>MVKVDLESKRYGEKLKEVFLMLDNNVVECIKEITESSRNGKLVFFVGAGVSTLSDYPQWWRLVDKYHEELYGSPKKGNYSSDEYLRIPQIFYNVKGEMAFDGILKDFFQVDKPTNPIHDKILAMNPAHVITTAYDNLIDTACWKRGKYFSVISAEEDVANATSSRYLLKVAGDFRKGFKGENVVLKEDDYLNYDQNYPLISNLMKTIIATHTIVFIGYGLGDYNINMLLNWVRKLQKDSFHKPFFIRTDPSPIENETLIYYENKGLRIIDAASLIDSNEYDYLERYSAVMDLLIESQENKFITKDDEVIDYIYGKISPLFALQYIRKIDLKHVFEYDYHFEVNGTVVRHKNKGFGYMERFFELKESCDERSKLSKKQYERFNALFNFFEKNGVICMAKDAGTLNTSIEINSLAYHGKYDVMKKFIEEQSVSIEDDYKKAFFLACLGRWEESYDLYSNIILNSIDESNGCVYYLSQINRYRIYQSITQAVTQFNGLGLLTFGRHYKPFTDEFLARIEREMTNFNIDDLFNGMPFEFQKKYKILEFLSDNQFLYDDTVKLFELTNKVRSEMSEGSYSFGMSSDIVVLLRLYDNLRFLYENCLWSVSFHEFHQYIRNSMSLLIEKAEYERTRDIDELGFSFFGKKSGFFMEYYDFVNISRHFKIDDIKNLERSCSIDKIRFGEQEKIEEYLVGIAEEITKQFSANGMNVVFYTQFISEAKAALYFAKYVKLSEEGLGKIVKALLFYFPERDLDIGKRYVWLERLTKCNELPKSIISIIDDFLVLQAEKHIDQNYSEVSSNGLYSRDYGALIKHFEKNFISKRLSEITLCLTQDKQKQIDFLFKLLPLLSTNAKSHLLSFKSVENINDLMNGIRIGLIDEFTPEHEELIIEYLETRKVNYIVEKEKGIQTFSSNDYMSTFGIWYFLEEINNSKMEEFIGMDDQYDFFVDPENFDYKKFIPSWLKNYNDKLLGKIAGNKHMKHHVIEVLKERVKNSNDKRYLEILMNYFI[4x];>MKTVIQDTADVYFK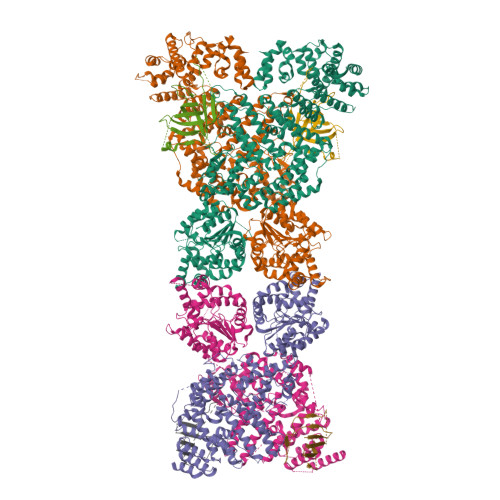RKSDGKLVFTAEAQTASFSQAISEEKLRGGIGNKPLYILKSEKEINLTVKNAFFDLEWLAMTQGETIQEETKVKVFDREHGLIVDDTNKVTLKGKPVSDVTFYNKKGLTYKIAVSTDGTYTIPTAFAAAKDKLTAVYQIEKVGRRLAIKASKFSERYEVEYRTIAYNPDTEEVYSDIYIQFPNVSPSGEFEMSLENGNALAPEIKFEALADTDTDEMAVVIEASRDENTAAPVEDTTGSTQSSDLGGTTE[4x]> MEDIKIKEIFENIYEVDLGDGLKRIATKSIVKGKKVYDEKIIKIGDEEYRIWNPNKSKLAAAIIKGLKVMPIKRDSKILYLGASAGTTPSHVADIADKGIVYAIEYAPRIMRELLDACAERENIIPILGDANKPQEYAN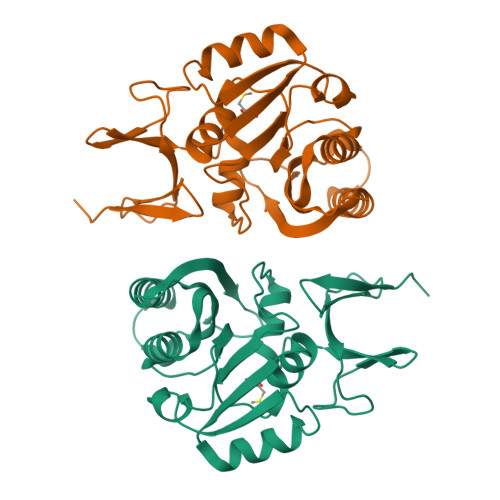IVEKVDVIYEDVAQPNQAEILIKNAKWFLKKGGYGMIAIKARSIDVTKDPKEIFKEQKEILEAGGFKIVDEVDIEPFEKDHVMFVGIWEGK>[2x]MEKVREIVREGIRVGNEDPRRIIHAFKVGLALVLVSSFYYYQPFGPFTDYFGINAMWAVATVVVVFEFSVGATLGKGLNRGVATLVAGGLGIGAHQLARLSGATVEPILLVMLVFVQAALSTFVRFFPWVKTKFDYGILIFILTFALISLSGFRDEEIMDLAESRLSTVVIGGVSCILISIFVCPVWAGQDLHSLLASNFDTLSHFLQDFGDEYFEAREKGDYKVVEKRKKNLERYKSVLDSKSDEEALANYAEWEPPHGQFRFRHPWKQYVAVGALLRQCAY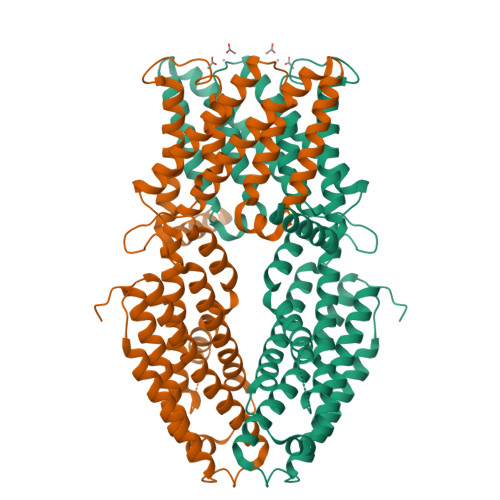RIDALNSYINSDFQIPVDIKKKLETPLRRMSSESGNSMKEMSISLKQMIKSSSSDIHVSNSQAACKSLSTLLKSGILNDVEPLQMISLMTTVSMLIDIVNLTEKISESVHELASAARFKNKMRPTVLYEKSDSGSIGRAMPIDSHEDHHVVTVLHDVDNDRSNNVDDSRGGSSQDSCHHVAIKIVDDNSNHEKHEDGEIHVHTLSNGHLQLEGGSSGGWSHPQFEK> QSGLQDGPEPTIHTQQAYAPEDDFTAKWTRADARQLQRMSDPTAPSRENSMPASVTMPTVPQDFPDMSNEQVWVWDTWPLTDEDANQYSVNGWEIIFSLVADRNLGFDDRHVFAKIGYFYRPAGVPAAERPENGGWTYGGLVFKE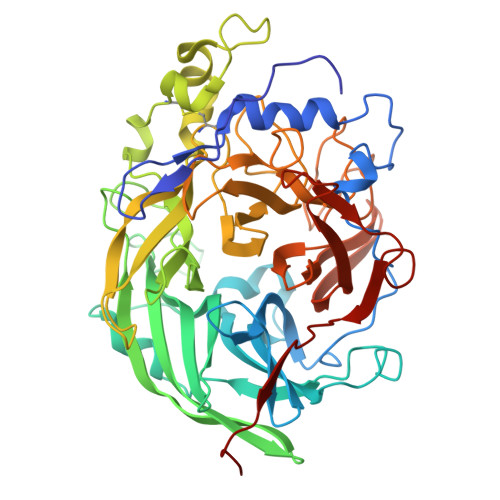GVTGQIFEDQSFSHQTQWSGSARVSKNGEIKLFFTDVAFYRNSDGTNIKPYDPRIALSVGKVKANKKGVTLTGFNKVTDLLQADGTYYQTGAQNEFFNFRDPFTFEDPAHPGETFMVFEGNSAMQRETATCNEADLGYRQGDPYAETVDDVNASGATYQIGNVGLAKAKNKQLTEWEFLPPILSANCVTDQTERPQIYFKDGKSYLFTISHRGTFAAGLDGPEGVYGFVGDGIRSDYQPLNGGSGLALGNPTNLNFLGGQPFAPDFNQHPGHFQAYSHYVMPGGLVQSFIDTIGTHDDFVRGGTLAPTVKMDIGVGGDPTKTAVDYSYGSEGLGGWADIPANKHLFTNGKF> MGTVSSRRSWWPLPLLLLLLLLLGPAGARAQEDEDGDYEELVLALRSEEDGLAEAPEHGTTATFHRCAKDPWRLPGTYVVVLKEETHLSQSERTARRLQAQAARRGYLTKILHVFHGLLPGFLVKMSGDLLELALKLPHVDYIEEDSSVFAQSIPWNLERITPPRYSADEYQPPDGGSLVEVYLLDTSIQSDHREIEGRVMVTDFENVPEEDGTRFHRQASKCDSHGTHLAGVVSGRDAGVAKGASMRSLRVLNCQGKGTVSGTLIG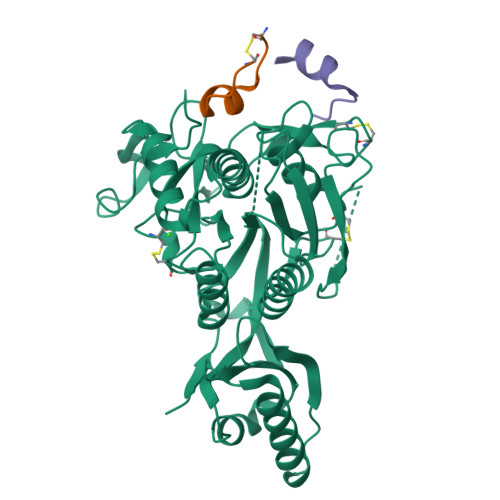LEFIRKSQLVQPVGPLVVLLPLAGGYSRVLNAACQRLARAGVVLVTAAGNFRDDACLYSPASAPEVITVGATNAQDQPVTLGTLGTNFGRCVDLFAPGEDIIGASSDCSTCFVSQSGTSQAAAHVAGIAAMMLSAEPELTLAELRQRLIHFSAKDVINEAWFPEDQRVLTPNLVAALPPSTHGAGNSHHHHHH;> CRLPWNLQRIGLPC;> XTVFTSWEEYLDWVX> MSSEDVKYFTRAEVAKNNTKDKNWFIIHNNVYDVTAFLNEHPGGEEVLIEQAGKDATEHFEDVGHSSDAREMMKQYKVGELVA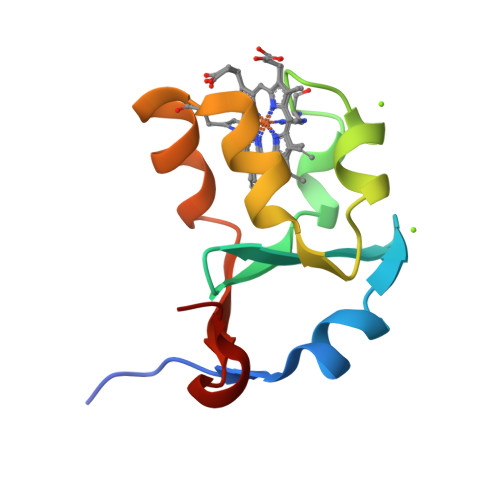EERSN>[2x]SMQLNQYTLKDEIGKGSYGVVKLAYNENDNTYYAMKVLSKKKLIRQAGFPRRPPPRGTRPAPGGCIQPRGPIEQVYQEIAILKKLDHPNVVKLVEVLDDPNEDHLYMVFELVNQGPVMEVPTLKPLSEDQARFYFQDLIKGIEYLHYQKIIHRDIKPSNLLVGEDGHIKIADFGVSNEFKGSDALLSNTVGTPAFMAPESLSETRKIFSGKALDVWAMGVTLYCFVFGQCPFMDERIMCLHSKI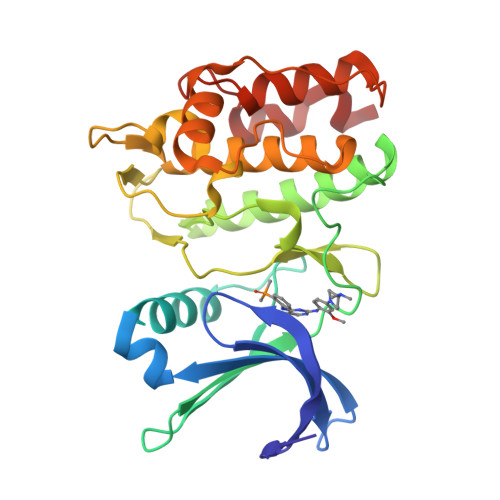KSQALEFPDQPDIAEDLKDLITRMLDKNPESRIVVPEIKLHPWVTRH>MTTGLSTAGAQDIGRSSVRPYLEECTRRFQEMFDRHVVTRPTKVELTDAELREVIDDCNAAVAPLGKTVSDERWISYVGVVLWSQSPRHIKDMEAFKAVCVLNCVTFVWDDMDPALHDFGLFLPQL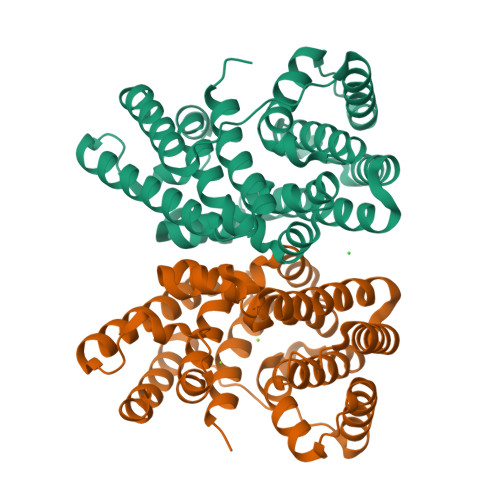RKICEKYYGPEDAEVAYEAARAFVTSDHMFRDSPIKAALCTTSPEQYFRFRVTDIGVDFWMKMSYPIYRHPEFTEHAKTSLAARMTTRGLTIVNDFYSYDREVSLGQITNCFRLCDVSDETAFKEFFQARLDDMIEDIECIKAFDQLTQDVFLDLIYGNFVWTTSNK[2x]>[4x]ASMTGGQQMGRDPGMTVTSQVKPEDEMDNWGRLILDGVSYSDMVGARDRPKEITWFDY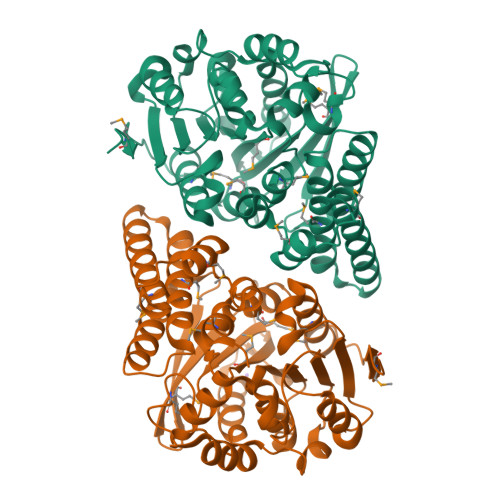WMSLANEYEQEAERKVALGHDLSAGELLMSAALCAQYAQFLWFDERRQKGQARKVELYQKAAPLLSPPAERHELVVDGIPMPVYVRIPEGPGPHPAVIMLGGLESTKEESFQMENLVLDRGMATATFDGPGQGEMFEYKRIAGDYEKYTSAVVDLLTKLEAIRNDAIGVLGRSLGGNYALKSAACEPRLAACISWGGFSDLDYWDLETPLTKESWKYVSKVDTLEEARLHVHAALETRDVLSQIACPTYILHGVHDEVPLSFVDTVLELVPAEHLNLVVEKDGDHCCHNLGIRPRLEMADWLYDVLVAGKKVAPTMKGWPLEHHHHHH>[2x]RSSQINDFKTIKMNHTNYLRNFFLQTTPETLESNLRDLLHSLEGESLNDLLALLLSEILSPGSQNLQNDPTRSWLTPPMVLDATNRGNVIARSISSLQANQINWNRVFNLMSTKYFLSAPLMPTTASLSCLFAALHDGPVIDEFFSCDWKVIFKLDLAIQLHKWSVQNGCFDLLNAEGTRKVSETIPNTKQSLLYLLSIASLNLELFLQREELSDGPMLAYFQECFFEDFNYAPEYLILALVKEMKRFVLLIENRTVIDEILITLLIQVHNKSPSSFKDVISTITDDSKIVDAAKIIINSDDAPIANFLKSLLDTGRLDTVINKLPFNEAFKILPCARQIGWEGFDTFLKTKVSPSNVDVVLESLEVQTKM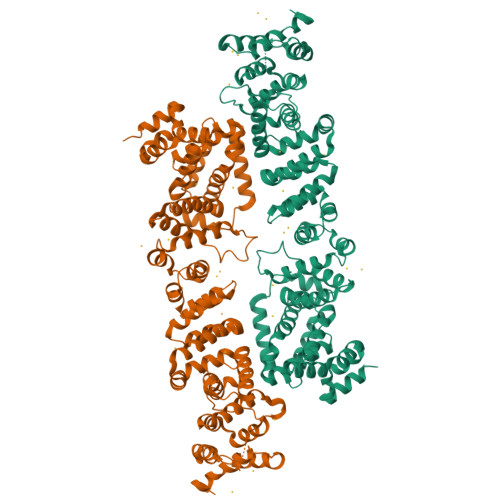TDTNTPFRSLKTFDLFAFHSLIEVLNKCPLDVLQLQRFESLEFSLLIAFPRLINFGFGHDEAILANGDIAGINNDIEKEMQNYLQKMYSGELAIKDVIELLRRLRDSDLPRDQEVFTCITHAVIAESTFFQDYPLDALATTSVLFGSMILFQLLRGFVLDVAFRIIMRFAKEPPESKMFKFAVQAIYAFRIRLAEYPQYCKDLLRDVPALKSQAQVYQSIVEAATLANAPKE2-amino-6-O-decanoyl-2-deoxy-beta-D-glucopyranose | 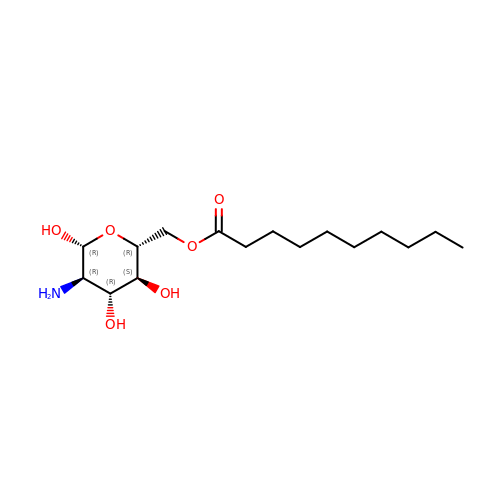C16 H31 N O6 | CEBTVLUOBKRBFG-JPIRQXTESA-N>MSLGNTTVVTTTVRNATPSLTL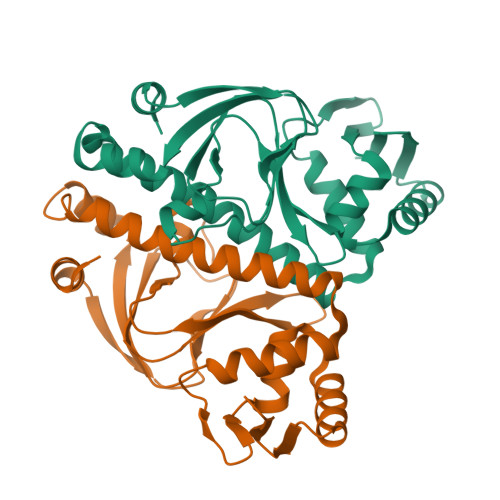DAGTIERFLAHSHRRRYPTRTDVFRPGDPAGTLYYVISGSVSIIAEEDDDRELVLGYFGSGEFVGEMGLFIESDTREVILRTRTQCELAEISYERLQQLFQTSLSPDAPRILYAIGVQLSKRLLDTTRKASRLAFLDVTDRIVRTLHDLSKEPEAMSHPQGTQLRVSRQELARLVGCSREMAGRVLKKLQADGLLHARGKTVVLYGTR[4x]> MKPMPLTLVEQILAEFQLQEEDLKKVMRRMQKEMDRGLRLETHEEASVKMLPTYVRSTPEGSEVGDFLSLDLGGTNFRVMLVKVGEGEEGQWSVKTK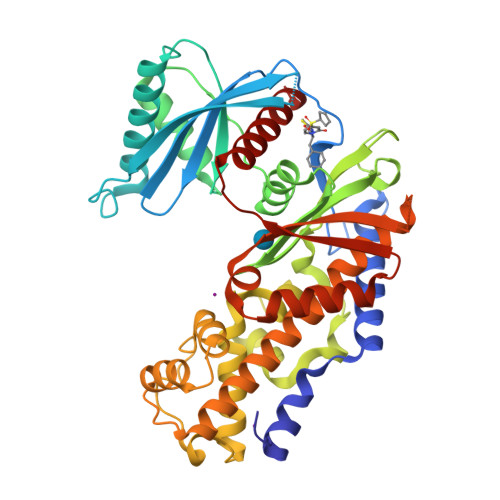HQMYSIPEDAMTGTAEMLFDYISECISDFLDKHQMKHKKLPLGFTFSFPVRHEDIDKGILLNWTKGFKASGAEGNNVVGLLRDAIKRRGDFEMDVVAMVNDTVATMISCYYEDHQCEVGMIVGTGCNACYMEEMQNVELVEGDEGRMCVNTEWGAFGDSGELDEFLLEYDRLVDESSANPGQQLYEKLIGGKYMGELVRLVLLRLVDENLLFHGEASEQLRTRGAFETRFVSQVESDTGDRKQIYNILSTLGLRPSTTDCDIVRRACESVSTRAAHMCSAGLAGVINRMRESRSEDVMRITVGVDGSVYKLHPSFKERFHASVRRLTPSCEITFIESEEGSGRGAALVSAVACKKACMLGQ> MKLGFVGAGRVGSTSAFTCLLNLDVDEIALVDIAEDLAVGEAMDLAHAAAGIDK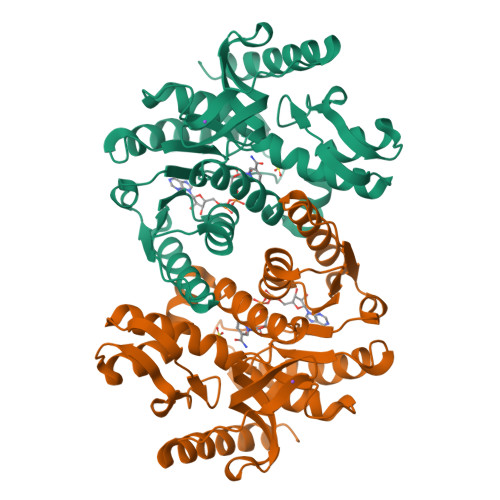YPKIVGGADYSLLKGSEIIVVTAGLARKPGMTRLDLAHKNAGIIKDIAKKIVENAPESKILVVTNPMDVMTYIMWKESGKPRNEVFGMGNQLDSQRLKERLYNAGARNIRRAWIIGEHGDSMFVAKSLADFDGEVDWEAVENDVRFVAAEVIKRKGATIFGPAVAIYRMVKAVVEDTGEIIPTSMILQGEYGIENVAVGVPAKLGKNGAEVADIKLSDEEIEKLRNSAKILRERLEELGY>[6x]MSLEENPAPDFTLN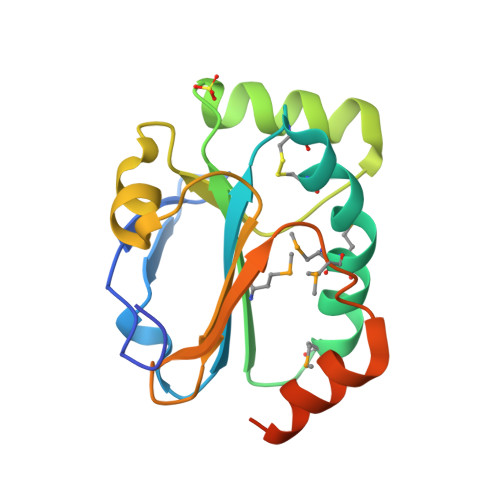TLNGEVVKLSDLKGQVVIVNFWATWCPPCREEIPSMMRLNAAMAGKPFRMLCVSIDEGGKVAVEEFFRKTGFTLPVLLDADKRVGKLYGTTGVPETFVIDRHGVILKKVVGAMEWDHPEVIAFLNNELSKAREGHHHHHH>GAASMEEPGAEEVRILFSTAKGESHTHKAGFKQLFRRLRSTYRPDKVDKDDFTLDTLRSAHILVLGGPKEKFTAPEVDMLKKFVKNGGSILILMSEGGEEKAGTNINYFLEQFGMSVNNDAVVRTTHYKYLHPKEVLISDGILNRAVITGAGKSLNSNDDDEFRVSRGPQAFDGTGLEYVFPFGATLSVQKPAVPVLSSGKIAYPMNRPVGAVWAQPGYGRIAVLGSCAMFDDKWLDKEENSKIMDFFFKFLEPHSKIQLN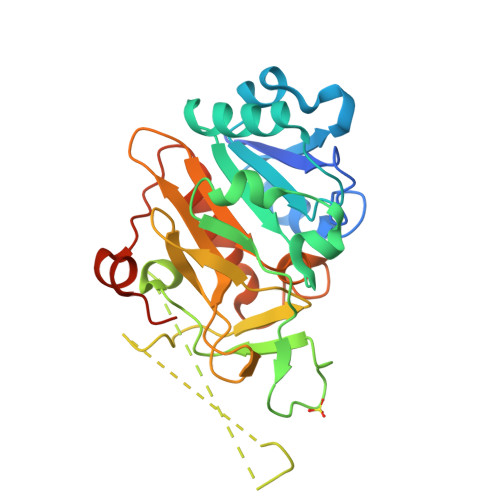DIDAEEPDVSDLKLLPDTA[3x]>MESYLVDTYQGIPYTAAVQVDLIEKDLLPASLTIWFPLFQANTPPAVLLDQLKTLTITTLYAASQNGPILKVNASAQGAAMSVLPKKFEVNATVALDEYSKLEFDKLTVCEVKTVYLTTMKPYGMVSKFVSSAKSVGKKTHDLIALCDFMDLEKNTPVTIPAFIKSVSIKESESATVEAAISSEADQALTQAKIAPYAGLIMIMTMNNPKGIFKKLGAGTQVIVELGAYVQAESISKICKTWSHQGTRYVLKSR[4x]

The matrix protein (M) of paramyxoviruses plays a key role in determining virion morphology by directing viral assembly and budding. The matrix protein (M) is a major component of the virus, and is thought to form an ordered layer beneath the viral membrane (Battisti et al., 2012; Liljeroos et al., 2013). M plays a critical role in assembly and budding through interactions with multiple viral and cellular components such as nucleoprotein-RNA oligomers (N-RNA; Ghildyal et al., 2002), lipid membranes (McPhee et al., 2011), and cytoplasmic tails of the viral glycoproteins (Henderson et al., 2002). We show that HMPV M is a dimer, both in the crystal and in solution, and Ca2+ stabilizes the structure.

In this study, we solved the X-ray crystallographic structure of the M protein from HMPV at 2.8 Å resolution. The P31 crystallographic asymmetric unit contains flattened, diamond-shaped M dimers. The M dimer is stabilized by a large network of conserved hydrophobic interactions with a buried interface area of 1,421 Å2 per monomer. Each M subunit is composed of two similarly folded domains (NTD and C-terminal domain [CTD]), which are joined by a 14-residue linker (residues 123–137) for which no density is visible. Each domain consists of a twisted β sandwich, in which the β strands in the opposing β sheets are approximately orthogonal to each other, and a few short α helices. CTD loops (residues 180–188 and residues 208–218) are not visible in the electron density, most probably due to intrinsic disorder in these regions. A unique feature of HMPV M among all experimentally solved M proteins so far is the presence of a Ca2+ binding site located on the solvent-exposed surface of the NTD. The binding pocket adopts the classic Ca2+ pentagonal bipyramidal geometry, with an average coordinating distance of 2.4 Å between Ca2+ and interacting oxygens. Binding involves the side chain carboxyls of Glu24 and Asp26, the backbone carbonyl of Leu28 and Lys101, and two water molecules. Dimers pack crystallographically through a relatively large (624 Å2) NTD/NTD interface that is stabilized by polar interactions, propagating a helical arrangement within the crystal.> GGUCAAGAUAGUAAGGGUCCACGGUGGAUGCCCUGGCGCUGGAGCCGAUGAAGGACGCGAUUACCUGCGAAAAGCCCCGACGAGCUGGAGAUACGCUUUGACUCGGGGAUGUCCGAAUGGGGAAACCCACCUCGUAAGAGGUAUCCGCAAGGAUGGGAACUCAGGGAACUGAAACAUCUCAGUACCUGAAGGAGAAGAAAGAGAAUUCGAUUCCGUUAGUAGCGGCGAGCGAACCCGGAUCAGCCCAAACCGAAACGCUUGCGUUUCGGGGUUGUAGGACCAGUUUUUAAGAUUCAACCCCUCAAGCCGAAGUGGCUGGAAAGCUACACCUCAGAAGGUGAGAGUCCUGUAGGCGAACGAGCGGUUGACUGUACUGGCACCUGAGUAGGUCGUUGUUCGUGAAACGAUGACUGAAUCCGCGCGGACCACCGCGCAAGGCUAAAUACUCCCAGUGACCGAUAGCGCAUAGUACCGUGAGGGAAAGGUGAAAAGAACCCCGGGAGGGGAGUGAAAGAGAACCUGAAACCGUGGACUUACAAGCAGUCAUGGCACCUUAUGCGUGUUAUGGCGUGCCUAUUGAAGCAUGAGCCGGCGACUUAGACCUGACGUGCGAGCUUAAGUUGAAAAACGGAGGCGGAGCGAAAGCGAGUCCGAAUAGGGCGGCAUUAGUACGUCGGGCUAGACUCGAAACCAGGUGAGCUAAGCAUGACCAGGUUGAAACCCCCGUGACAGGGGGCGGAGGACCGAACCGGUGCCUGCUGAAACAGUCUCGGAUGAGUUGUGUUUAGGAGUGAAAAGCUAACCGAACCUGGAGAUAGCUAGUUCUCCCCGAAAUGUAUUGAGGUACAGCCUCGGAUGUUGACCAUGUCCUGUAGAGCACUCACAAGGCUAGGGGGCCUACCAGCUUACCAAACCUUAUGAAACUCCGAAGGGGCACGCGUUUAGUCCGGGAGUGAGGCUGCGAGAGCUAACUUCCGUAGCCGAGAGGGAAACAACCCAGACCAUCAGCUAAGGUCCCUAAAUGAUCGCUCAGUGGUUAAGGAUGUGUCGUCGCAUAGACAGCCAGGAGGUUGGCUUAGAAGCAGCCACCCUUCAAAGAGUGCGUAAUAGCUCACUGGUCGAGUGACGAUGCGCCGAAAAUGAUCGGGGCUCAAGUGAUCUACCGAAGCUAUGGAUUCAACUCGCGAAGCGAGUUGUCUGGUAGGGGAGCGUUCAGUCCGCGGAGAAGCCAUACCGGAAGGAGUGGUGGAGCCGACUGAAGUGCGGAUGCCGGCAUGAGUAACGAUAAAAGAAGUGAGAAUCUUCUUCGCCGUAAGGACAAGGGUUCCUGGGGAAGGGUCGUCCGCCCAGGGAAAGUCGGGACCUAAGGUGAGGCCGAACGGCGCAGCCGAUGGACAGCAGGUCAAGAUUCCUGCACCGAUCAUGUGGAGUGAUGGAGGGACGCAUUACGCUAUCCAAUGCCAAGCUAUGGCUAUGCUGGUUGGUACGCUCAAGGGCGAUCGGGUCAGAAAAUCUACCGGUCACAUGCCUCAGACGUAUCGGGAGCUUCCUCGGAAGCGAAGUUGGAAACGCGACGGUGCCAAGAAAAGCUUCUAAACGUUGAAACAUGAUUGCCCGUACCGCAAACCGACACAGGUGUCCGAGUGUCAAUGCACUAAGGCGCGCGAGAGAACCCUCGUUAAGGAACUUUGCAAUCUCACCCCGUAACUUCGGAAGAAGGGGUCCCCACGCUUCGCGUGGGGCGCAGUGAAUAGGCCCAGGCGACUGUUUACCAAAAUCACAGCACUCUGCCAACACGAACAGUGGACGUAUAGGGUGUGACGCCUGCCCGGUGCCGGAAGGUCAAGUGGAGCGGUGCAAGCUGCGAAAUGAAGCCCCGGUGAACGGCGGCCGUAACUAUAACGGUCCUAAGGUAGCGAAAUUCCUUGUCGGGUAAGUUCCGACCUGCACGAAAGGCGUAACGAUCUGGGCGCUGUCUCAACGAGGGACUCGGUGAAAUUGAAUUGGCUGUAAAGAUGCGGCCUACCCGUAGCAGGACGAAAAGACCCCGUGGAGCUUUACUAUAGUCUGGCAUUGGGAUUCGGGUUUCUCUGCGUAGGAUAGGUGGGAGCCUGCGAAACUGGCCUUUUGGGGUCGGUGGAGGCAACGGUGAAAUACCACCCUGAGAAACUUGGAUUUCUAACCUGAAAAAUCACUUUCGGGGACCGUGCUUGGCGGGUAGUUUGACUGGGGCGGUCGCCUCCCAAAAU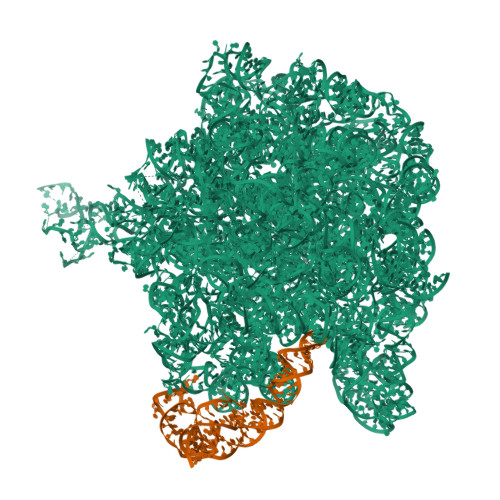GUAACGGAGGCGCCCAAAGGUCACCUCAAGACGGUUGGAAAUCGUCUGUAGAGCGCAAAGGUAGAAGGUGGCUUGACUGCGAGACUGACACGUCGAGCAGGGAGGAAACUCGGGCUUAGUGAACCGGUGGUACCGUGUGGAAGGGCCAUCGAUCAACGGAUAAAAGUUACCCCGGGGAUAACAGGCUGAUCUCCCCCGAGAGUCCAUAUCGGCGGGGAGGUUUGGCACCUCGAUGUCGGCUCGUCGCAUCCUGGGGCUGAAGAAGGUCCCAAGGGUUGGGCUGUUCGCCCAUUAAAGCGGCACGCGAGCUGGGUUCAGAACGUCGUGAGACAGUUCGGUCUCUAUCCGCUACGGGCGCAGGAGAAUUGAGGGGAGUUGCUCCUAGUACGAGAGGACCGGAGUGAACGGACCGCUGGUCUCCCUGCUGUCGUACCAACGGCACAUGCAGGGUAGCUAUGUCCGGAACGGAUAACCGCUGAAAGCAUCUAAGCGGGAAGCCAGCCCCAAGAUGAGUUCUCCCACUGUUUAUCAGGUAAGACUCCCGGAAGACCACCGGGUUAAGAGGCCAGGCGUGCACGCAUAGCAAUGUGUUCAGCGGACUGGUGCUCAUCAGUCGAGGUCUUGACCACUC;> CCCCCGUGCCCAUAGCACUGUGGAACCACCCCACCCCAUGCCGAACUGGGUCGUGAAACACAGCAGCGCCAAUGAUACUCGGACCGCAGGGUCCCGGAAAAGUCGGUCAGCGCGGGGG> MKQSEFRRWLESQGVDVANGSNHLKLRFHGRRSVM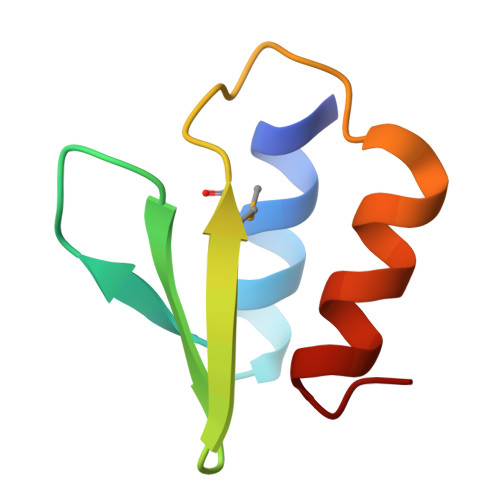PRHPCDEIKEPLRKAILKQLGLS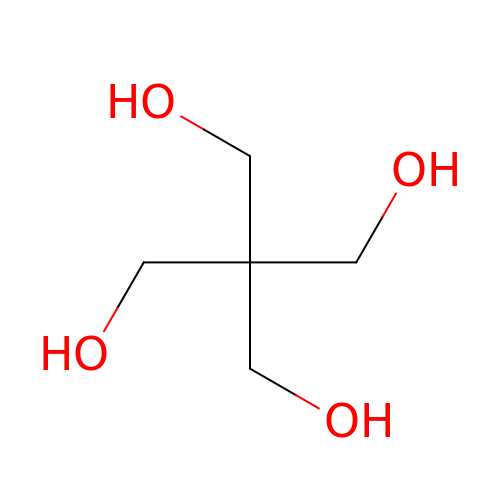2,2-bis(hydroxymethyl)propane-1,3-diol | C5 H12 O4 | WXZMFSXDPGVJKK-UHFFFAOYSA-N>GPMFQRSTPAITLESPDIKYPLRLIDREIISHDTRRFRFALPSPQHILGLPVGQHIYLSARIDGNLVVRPYTPISSDDDKGFVDLVIKVYFKDTHPKFPAGGKMSQYLESMQIGDTIEFRGPSGLLVYQGKGKFAIRPDKKSNPIIRTVKS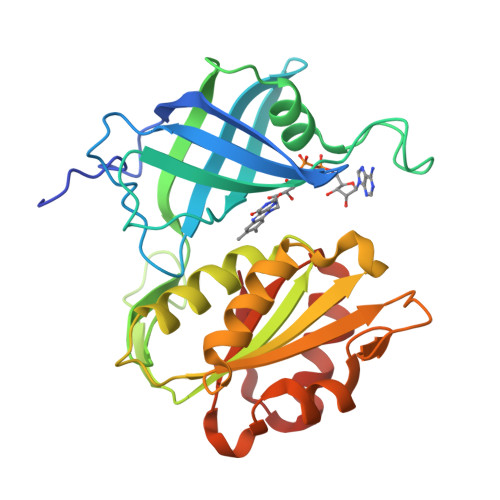VGMIAGGTGITPMLQVIRAIMKDPDDHTVCHLLFANQTEKDILLRPELEELRNKHSARFKLWYTLDRAPEAWDYGQGFVNEEMIRDHLPPPEEEPLVLMCGPPPMIQYACLPNLDHVGHPTERCFVF[5x]> GPGMAVKHLIVLKFKDEITEAQKEEFFKTYVNLVNIIPAMKDVYWGKDVTQKNKEEG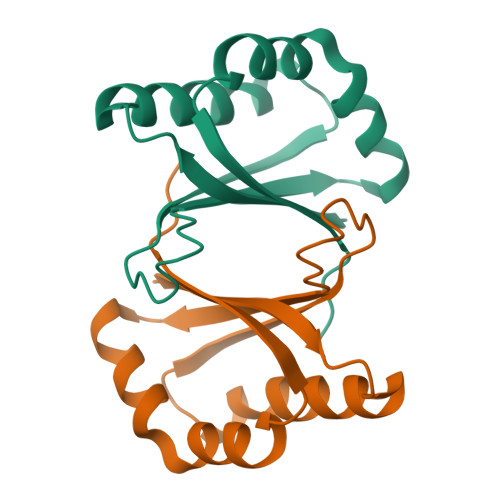YTHIVEVTFESVETIQDYIIHPASVGFGDVYRSFWEKLLIFDYTPRK>[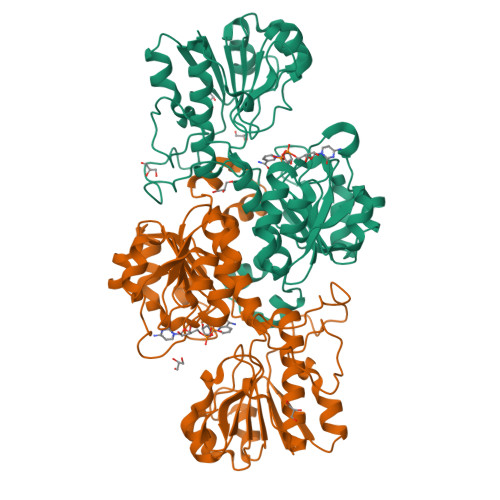2x]MAKVLCVLYDDPVDGYPKTYARDDLPKIDHYPGGQTLPTPKAIDFTPGQLLGSVSGELGLRKYLESNGHTLVVTSDKDGPDSVFERELVDADVVISQPFWPAYLTPERIAKAKNLKLALTAGIGSDHVDLQSAIDRNVTVAEVTYCNSISVAEHVVMMILSLVRNYLPSHEWARKGGWNIADCVSHAYDLEAMHVGTVAAGRIGLAVLRRLAPFDVHLHYTDRHRLPESVEKELNLTWHATREDMYPVCDVVTLNIPLHPPTEHMINDETLKLFKRGAYIVNTARGKLCDRDAVARALESGRLAGYAGDVWFPQPAPKDHPWRTMPYNGMTPHISGTTLTAQARYAAGTREILECFFEGRPIRDEYLIVQGGALAGTGAHIYSKGNATGGSEEAAKFKKAV>MHHHHHHTPTAQTTASARRVVFPFTAIVGQEEMKLALLLNVIDPKIGGVMIMGDRGTGKSTTIRALADLLPEIPVVANDPFNSDPSDPDLMSDEVRQKSGTGAEIPIEFKKVQMVDLPLGATEDRVCGTIDIEKALSEGVKAFEPGLLAKANRGILYVDEVNLLDDHLVDVLLDSAASGWNTVEREGISIRHPARFVLVGSGNPEEGELRPQLLDRFGMHAEIHTVKEPALRVQIVEQRSEFDQNPPTFLEKYNPEQTALQKKIVEAQKLLPEVKLDYDLRVKISEVCSELDVDGLRGDIVTNRAAKALTAYEGRTEVTVDDIRRVITLCLRHRLRKDPLESIDSGYKVEKVFARIFGVELLEDDSSQKNGAGQIKTGVR[6x]

Magnesium chelatase is a conserved enzyme complex responsible for the first committed step of chlorophyll biosynthesis in photosynthetic organisms, which is the addition of magnesium to the chlorophyll precursor, protoporphyrin IX. The complex is composed of the catalytic subunit ChlH, the bridging subunit ChlD, and the subunit ChlI, which serves as the motor that drives the entire complex. The motor subunit ChlI belongs to the superfamily of AAA+ (ATPases associated with diverse cellular activities) proteins and, through binding and hydrolyzing of ATP, provides the energy for the thermodynamically unfavorable reaction of Mg2+ insertion into protoporphyrin IX. Here, we used a combination of cryo-EM and functional analysis to investigate the mechanism of the ChlI motor subunit of magnesium chelatase from the cyanobacterium Nostoc sp. PCC 7120 (hereafter, Nostoc).

Iterative rounds of 3D classification, performed by multiple-class ab initio reconstructions followed by heterogeneous refinements, revealed two distinct classes, which we named hexamer conformations A and B. These reconstructions achieved global resolutions of 4 Å and 3.8 Å, respectively, with much greater local resolutions in the central parts of the structures. Conformation A is characterized by ATP molecules bound in five monomers and ADP in one, while conformation B has ATP bound in four monomers and ADP in two. Interestingly, each monomer contains a bound nucleotide molecule (ATP or ADP) in both hexameric states. The Nostoc ChlI hexameric ring conformations have diameters of approximately 114–117 Å, with a central pore of about 33 Å. In the hexamer structures, the nucleotide state of each monomer is related to the structural organization of the insertions of that monomer, such that when an ATP molecule is bound, the insertions are folded and in an upward position. If ADP is bound, the inserts of this monomer are more flexible or even unfold, as demonstrated by fuzzy or absent corresponding cryo-EM densities. Interestingly, in the observed ADP-bound states, the side chains of the adjacent R210 arginine fingers are positioned somewhat away from the nucleotide (inset 5), in line with data from other AAA+ proteins. Arginine finger R210 and sensor 2 R291 residues from the adjacent monomer additionally coordinate the nucleotide molecule and contribute to the inter-subunit cooperation within the hexamer, which is typical for AAA+ proteins. Not only the structured inserts undergo conformational changes upon ATP hydrolysis in ChlI but also the whole hexamer ring experiences rigid-body rearrangements apparently caused by the ATP hydrolysis-induced reorganization of key amino-acid residues in close proximity to the nucleotide-binding pocket. According to our model, ATP hydrolysis occurs in one monomer at a time, triggering rearrangements involving residues near the nucleotide-binding pocket.> MSDKIIHLTDDSFDTDVLKADGAILVDFWAEWCGPCKMIA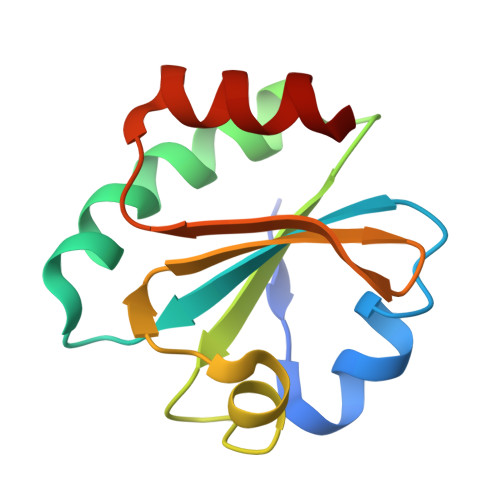PILDEIADEYQGKLTVAKLNIDQNPGTAPKYGIRGIPTLLLFKNGEVAATKVGALSKGQLKEFLDANLA>RMEIVKIPVVVHVVW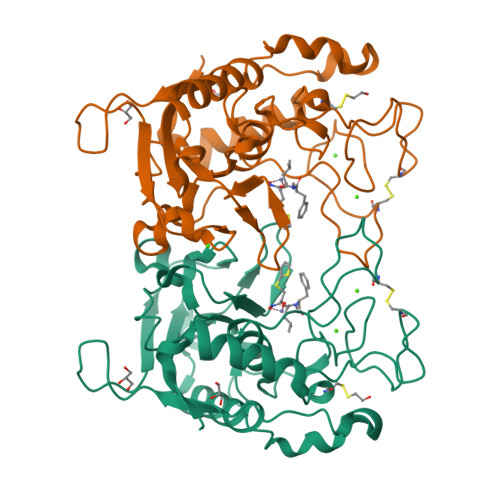NEEEENISDAQIQSQIDILNKDFRKLNSDVSQVPSVWSNLIADLGIEFFLATKDPNGNQTTGITRTQTSVTFFTTSDEVKFASSGGEDAWPADRYLNIWVCHVLKSEIGQDILGYAQFPGGPAETDGVVIVDAAFGTTGTALPPFDKGRTATHEIGHWLNLYHIWGDELRFEDPCSRSDEVDDTPNQADPNFGAPSYPHVSCSNGPNGDMFMNYMDYVDDKCMVMFTQGQATRVNACLDGPRSSFLA[2x]>GHMKCPVCHQGEMVSGIKDIPYTFRGRKTVLKGIHGLYCVHCEESIMNKEESDAFMAQVKAFRASVNAETVAPEFIVKVRKKLSLTQKEASEIFGGGVNAFSRYEKGNAQPHPSTIKLLRVLDKHPELLNEIR[2x]

Our biochemical and structural analysis of the E. coli MqsA antitoxin and the MqsR:MqsA-N complex provide a detailed 3-dimensional structural view of the free antitoxin and the TA complex. These structures combined with our biochemical data unequivocally demonstrate that MqsR, a protein previously shown to be critical for biofilm formation and the most highly upregulated gene in persister cells in E. coli, and MqsA form a novel bacterial TA system. Our data show that, as expected for a TA system, the expression of the MqsR toxin leads to growth arrest, while co-expression with its antitoxin, MqsA, rescues the growth arrest phenotype. In addition, MqsR associates with MqsA to form a tight, non-toxic complex and both MqsA alone and the MqsR:MqsA2:MqsR complex bind and regulate the mqsR promoter. MqsA itself is a two-domain protein with a novel fold that, unlike every other antitoxin, is well-ordered throughout its entire sequence and whose structure does not change upon toxin binding.

MqsA-F was determined to a resolution of 2.15 Å by molecular replacement using the structures of the MqsA N-terminal domain (residues 1–76, referred to hereafter as MqsA-N) and the MqsA C-terminal domain (residues 62–131; referred to hereafter as MqsA-C), as search models. The space group of the MqsA-F crystal is P21, with two molecules in the asymmetric unit. The two monomers are identical in terms of the overall fold with well-ordered electron density throughout both chains. The final model contains 262 residues, and includes all 131 residues for each MqsA-F molecule. The MqsA monomer is composed of two structurally distinct domains connected by a flexible linker and resembles a human leg: the MqsA-N, composed of residues 1–67, is the ‘foot’ and ‘calf’ and the MqsA-C, composed of residues 69–131, is the ‘thigh’. The ‘knee’-like linker connecting the domains, centered on residue 68, is flexible, allowing the N- and C-terminal domains to rotate independently of one another as rigid bodies (superposition of the N- and C-terminal domains from chains A and B give RMSD values of 0.35 Å and 0.58 Å, respectively). Superposition of the C-terminal domains from both monomers shows that the corresponding N-terminal domains are rotated by ∼25° with respect to one another. MqsA dimerization is mediated by the MqsA-C HTH-XRE domain. Residues from α-helices 3, 5, and 6 participate in the dimerization interface, which buries 1600 Å2 of solvent accessible surface area (SASA; this constitutes 19.9% of the total SASA) and has a surface complementarity of 0.69, both of which are well within the ranges expected for biologically relevant protein:protein interactions. Six residues are buried upon dimer formation, including Ser112, Lys115, Leu116, Val119, Leu126 and Ile130.>MVTVGNYCEAEGPVGPAWMQDGLSPCFFFTLVPSTRMALGTLALVLALPCRRRERPAGADSLSWGAGPRISPYVLQLLLATLQAALPLAGLAGRVGTARGAPLPSYLLLASVLESLAGACGLWLLVVERSQARQRLAMGIWIKFRHSPGLLLLWTVAFAAENLALVSWNSPQWWWARADLGQQVQFSLWVLRYVVSGGLFVLGLWAPGLRPQSYTLQVHEEDQDVERSQVRSAAQQSTWRDFGRKLRLLSGYLWPRGSPALQLVVLICLGLMGLERALNVLVPIFYRNIVNLLTEKAPWNSLAWTVTSYVFLKFLQGGGTGSTGFVSNLRTFLWIRVQQFTSRRVELLIFSHLHELSLRWHLGRRTGEVLRIADRGTSSVTGLLSYLVFNVIPTLADIIIGIIYFSMFFNAWFGLIVFLCMSLYLTLTIVVTEWRTKFRRAMNTQENATRARAVDSLLNFETVKYYNAESYEVERYREAIIKYQGLEWKSSASLVLLNQTQNLVIGLGLLAGSLLCAYFVTEQKLQVGDYVLFGTYIIQLYMPLNWFGTYYRMIQTNFIDMENMFDLLKEETEVKDLPGAGPLRFQKGRIEFENVHFSYADGRETLQDVSFTVMPGQTLALVGPSGAGKSTILRLLFRFYDISSGCIRIDGQDISQVTQASLRSHIGVVPQDTVLFNDTIADNIRYGRVTAGNDEVEAAAQAAGIHDAIMAFPEGYRTQVGERGLKLSGGEKQRVAIARTILKAPGIILLDQATSALDTSNERAIQASLAKVCANRTTIVVAHRLSTVVNADQILVIKDGCIVERGRHEALLSRGGVYADMWQLQQGQEETSEDTKPQTMER[2x]

ABCB6 is an 842-amino acid protein that belongs to the B subfamily of the ABC transporter. ABCB6 is a “half-transporter” that contains a single pair of TMD and NBD, but needs to form a homodimer to be functional. ABCB6 is a porphyrin transporter located in the outer membrane of mitochondria that may regulate the heme biosynthetic pathway together with the plasma membrane porphyrin transporter ABCG216,17. ABCB6 plays a crucial role in energy-dependent porphyrin transport, drug resistance, toxic metal resistance, porphyrin biosynthesis, protection against stress, and encoding a blood group system Langereis antigen.

Furthermore, we solved the nucleotide-bound structure of human hABCB6[EQ] at 3.5-Å resolution by using cryo-EM, allowing for unambiguous side-chain placement for most of the protein. The nucleotide-bound hABCB6[EQ] forms an occluded conformation compared with the apo-state inward-facing conformation. The remarkable change between nucleotide-bound state and apo-state is the closure of opposing NBDs triggered by the binding of ATP and Mg2+. The closure of the two NBDs leads to an anticlockwise rotation of TM4 and 5, which is a common feature of conformational change within ABC transporters. In the lipid bilayer, the closure of the two NBDs also triggers the rotation of the plug to eliminate the barrier for substrate translocation and the TMDs adopt a collapsed conformation without substrate binding. In the nucleotide-bound structure, the “plug” swinging to TM6 belongs to the same monomer to form an open state and clears a pathway toward the outside, accompanied by the conformational change of the two W546 residues and forming π–π interaction to further constitute a “bottom” of the cavity 2. In this process, the “H–P” cavity 1 disappears and cavity 2 is decreased to extrude substrates. The differences between these two conformations in the TMD are the decreases of cavities 1 and 2 in the occluded conformation, as well as a slight opening of the extracellular vestibule. Our nucleotide-bound structure reveals a substrate-free conformation, despite the incubation of 20 μM PPIX with the protein before cryo-EM sample preparation. The structure indicates that cavity 2 of hABCB6 is not suitable for the accommodation of substrates in this state and substrates escaped from this cavity before the hydrolysis of ATP.> 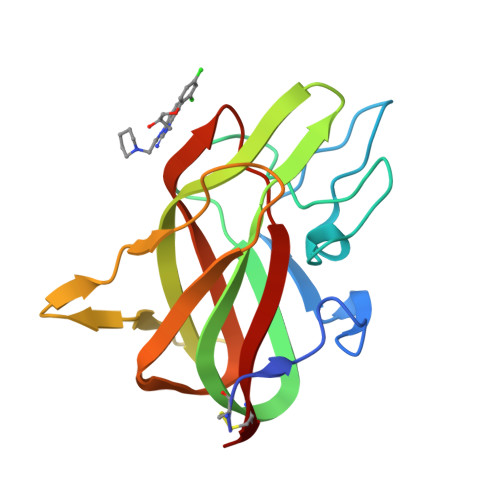DLNSCSMPLGMESKAISDAQITASSYFTNMFATWSPSKARLHLQGRSNAWRPQVNNPKEWLQVDFQKTMKVTGVTTQGVKSLLTSMYVKEFLISSSQDGHQWTLFFQNGKVKVFQGNQDSFTPVVNSLDPPLLTRYLRIHPQSWVHQIALRMEVLGCEA>MGHHHHHHGGVKKELSNSKKIEDQSRESVLSDISSRTLAFPSISTADFQFDLDRASDIIVDAVADILQKYDNIRLVLVDLSHKSRILSLVKEKAAKKNINSSRFFTFVGDITQLQSKGGLRCNVIANAANWRLKPGGGGVNAAIYNAAGEDLQRATKECAD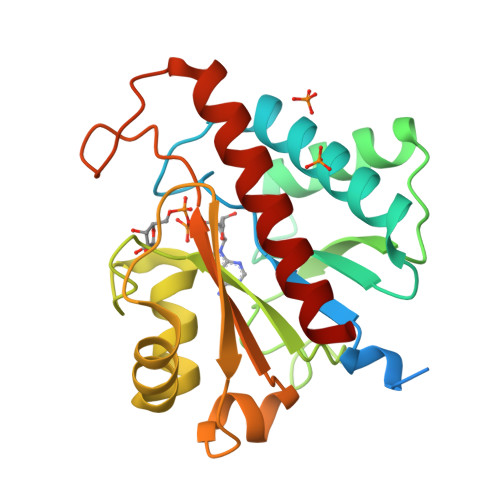TLRPGSSVAVPLPSTSPLHQREGVTHIIHVLGPNMNPMRPDCLKNDYTKGSKILHEAYTSLFENFVAIVQ[2x]> MSATKSIVGEALEYVNIGLSHFLALPLAQRISLIIIIPFIYNIVWQLLYSLRKDRPPLVFYWIPWVGSAVVYGMKPYEFFEECQKKYGDIFSFVLLGRVMTVYLGPKGHEF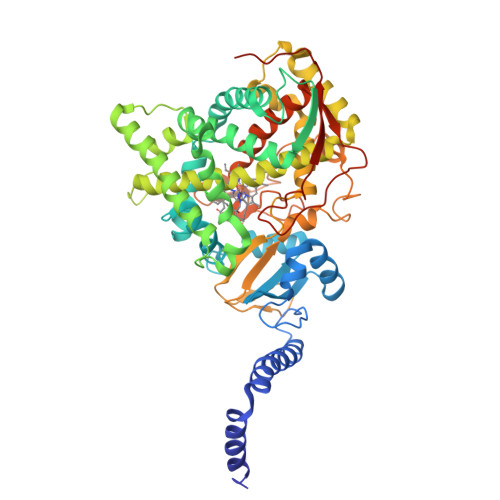VFNAKLADVSAEAAYAHLTTPVFGKGVIYDCPNSRLMEQKKFVKGALTKEAFKSYVPLIAEEVYKYFRDSKNFRLNERTTGTIDVMVTQPEMTIFTASRSLLGKEMRAKLDTDFAYLYSDLDKGFTPINFVFPNLPLEHYRKRDHAQKAISGTYMSLIKERRKNNDIQDRDLIDSLMKNSTYKDGVKMTDQEIANLLIGVLMGGQHTSAATSAWILLHLAERPDVQQELYEEQMRVLDGGKKELTYDLLQEMPLLNQTIKETLRMHHPLHSLFRKVMKDMHVPNTSYVIPAGYHVLVSPGYTHLRDEYFPNAHQFNIHRWNNDSASSYSVGEEVDYGFGAISKGVSSPYLPFGGGRHRCIGEHFAYCQLGVLMSIFIRTLKWHYPEGKTVPPPDFTSMVTLPTGPAKIIWEKRNPEQKIGGRHHHHHH>MSLKTTLPISLDWSTEEVIDVVHFFQAIEQAYDQGIAREDLLGKYRRFKEIVPSKSEEKQLFRAYEQENDVSCYQTIKKAREEMEEHIQMEGHHHHHH[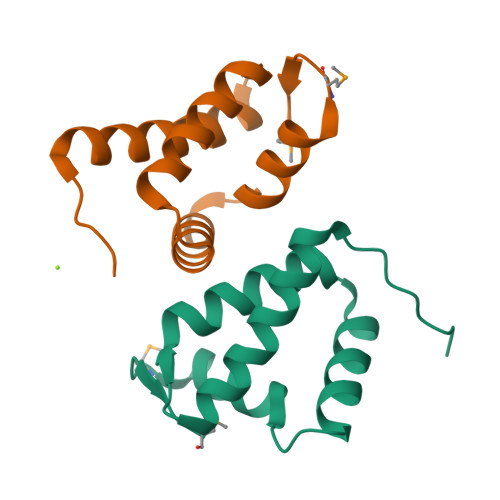2x]>[2x]MAGSSEEAPDYGRGVVIMDDWPGYDLNLFTYPQHYYGDLE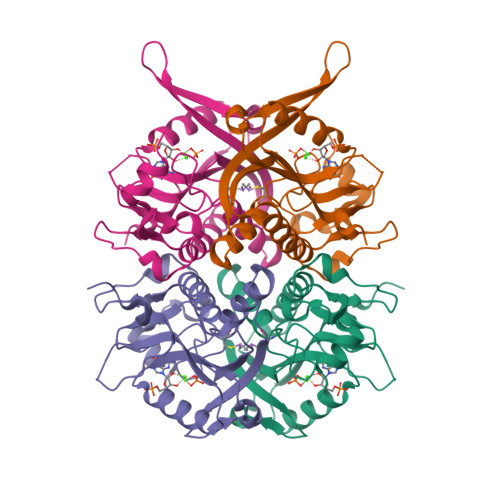YVLIPHGIIVDRIERLAKDIMKDIGYSDIMVLCVLKGGYKFCADLVEHLKNISRNSDRFVSMKVDFIRLKSYRNDQSMGEMQIIGGDDLSTLAGKNVLIVEDVVGTGRTMKALLSNIEKYKPNMIKVASLLVKRTSRSDGFRPDYAGFEIPNLFVVGYALDYNEYFRDLNHICVINEHGKEKYRV>GASGSEIPKIQPFFFPKNLTTGKTVKVICNPSEGSLPFTFEWLKDGTQVVPSAHVAVKTHEDYSLLNIDSVGWEDAGNYSCVLNNSAGSDTHTATLSVFA[2x]

Recently, a shortened Dscam (sDscam) gene family with tandemly arrayed 5′ cassettes in Chelicerata species has been identified, which encodes ∼50–100 isoforms. Chelicerata sDscams could be classified into two subfamilies, sDscamα and sDscamβ, containing one and two variable Ig domains, respectively. Crystal structures and cell aggregation assays demonstrated that both α and β subfamilies of sDscam used Ig1 for the isoform-specific trans recognition in a hand-in-hand manner. Furthermore, the cis interactions were established by the three FNIII domains of sDscam, which assemble into a cross fold with a kink between FNIII2 and FNIII3.

To elucidate the molecular details of trans interactions of sDscam, we determined the crystal structures of Ig1 from Mesobuthus martensii sDscam isoforms α1, α7, and β6v2. We also determined the crystal structures of sDscam Ig1 from another chelicerate species Limulus polyphemus (isoforms α7 and β3v7) to provide insights into the conservation of sDscam trans recognition within Chelicerata. These crystal structures of Ig fragments were determined at 1.3–3.1 Å resolutions. The crystal structures of sDscam Ig1 from both M. martensii and L. polyphemus revealed a common assembly of antiparallel homodimer for both α and β subfamilies of sDscam. A previous study has demonstrated that Drosophila Dscam1 Ig7 use its ABED face to form a homophilic dimer through a charge complementary mechanism to ensure an antiparallel binding mode. Similarly, sDscam Ig1 also employs the ABED face to form an antiparallel homodimer. However, among the seven Ig1 structures reported here, the complementary electrostatic potential surface pattern (negative in one end, neutral in the middle, and positive in the other end) has been only observed in the three β isoforms, but not in any one of the four α isoforms. Electrostatic and shape complementarity had been observed in all Ig1 dimer interfaces.>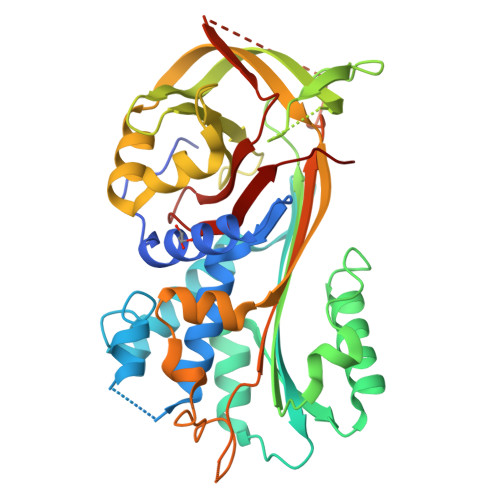MGHHHHHHGQQDVHGPFQGQRQNEFDLMFVKEIFKNHNSNVVLSPFSVKILLTLIYEASDTSFGNAVSNTKRELSSVIQNDNIDHTRSYYKQLLESAQQDNKDYDLNIATNFFVDDFIEVINKYQQIANTHYHAMLEKVSYSNPTQTAATINNWVSEHTNGRLREIVTPDSLEGAVITLVNVIYFKGLWTYPFPEVANNVKPFYGTRGKPTNAQYMEQNGQFYYDNSADLGAQILRLPYRGNKLAMYFILPNPDNTVNQVLDRINSASLHQALWYMEENEVNVTLPKFKFDFSEQLNEPLQQVGIREIFSQNASLPLLARGRGARDEVRVSRIFQKAGITINELGEEAYAATEIQLVNKFGGDGVQIFNANRPFIFFIEDETLGTMLFAGKIENPVF[3x]> GPLGSRLKYPVSQQNKNAPSTAGLGYGSWEIDPKDLTFLKELGTGQFGVVKYGKWRGQYDVAIKMIKEGSMSEDEFIEEAKVMMNLSHEKL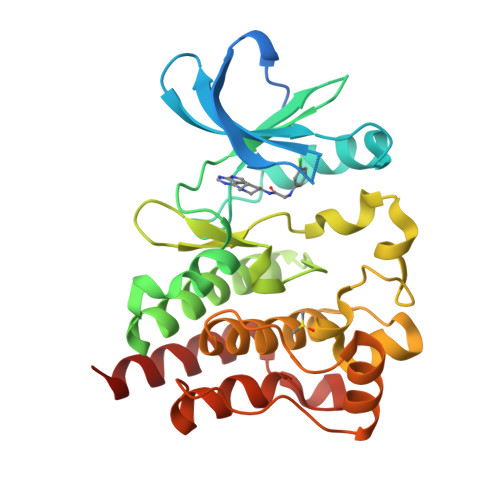VQLYGVCTKQRPIFIITEYMANGCLLNYLREMRHRFQTQQLLEMCKDVCEAMEYLESKQFLHRDLAARNCLVNDQGVVKVSDFGLSRYVLDDEYTSSVGSKFPVRWSPPEVLMYSKFSSKSDIWAFGVLMWEIYSLGKMPYERFTNSETAEHIAQGLRLYRPHLASEKVYTIMYSCWHEKADERPTFKILLSNILDVMDEES>MQLFHKAINRRGTHSIKWDTYKNEELIHAWIADMDFEVPKPIQTALKQRIKHPIFGYTLPPENIGDIICNWTKQQYDWDIQKEWIVFSAGIVPALSTSIQAFTKENESVLVQPPIYPPFFEMVTTNNRQLCVSPLQKQNDTYVIDFKHLEKQFQQGIKLMLLCSPHNPIGRVWTKEELIKLGSLCTKYNVIVVADEIHSDIIYADHTHTPFASLSEELAERTITCMAPSKTFNIAGLQASIIIIPNEKLRHAFTAIQYRQGFHGLNIFAYTAMQSAYTECNDWLNKIRLYIEDNAKFACEYMKDHIPTLSVTKPEGSFLLWI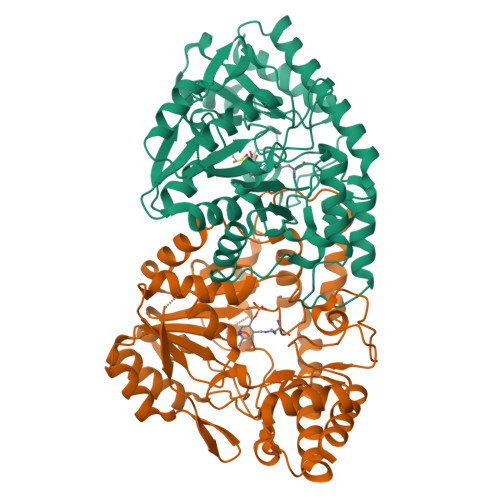DCSALNLSQDERTKLLEEKGKIIVEPGEKYGLGGEEHIRINIGCPRSVLEEILNRLRHTFS[2x]(5alpha,8alpha)-17-(pyridin-3-yl)androst-16-en-3-one | C24 H31 N 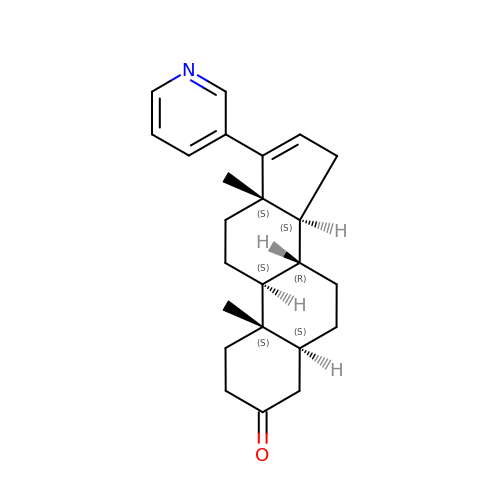O | FKNZCFYWNHCQGE-IRMBCWQZSA-N>LTVNGDRLWDSLMDMAKIGPGIAGGNNRRTLTDEDAEGRRLFQRWCEAAGLTMGVDRMGTMFATRPGEDPEALPVYIGSHLDTQPTGGKFDGVLGVLAGLEVVRSLNDLNIKTKHPIVVTNWSNEEGARFAPAMLASGVFAGIHDLDYAYSRTDTDGKTYGEELKRIGWLGEEEVGARRMHAYFEYHIEQGPILEADGKQIGVVTHGQGLWWLEVTLTGKEAHTGSTPMAMRVNAGLAAARILEKVQEVAMAHQPGAVAGVGQMIFTPNSRNVLPGKVVFTIDLRTPSQAKLDSMRAIFEREVPAIAEELGVGCSIEAIGHFDPVTFDAVLVGRVRAAAERLGYSHMDIISGAGHDACWTARVAPSTMIFCPCVDGLSHNEAEEISPEWAAAGCDVLLHAVLETAEIVQ[2x]

N‐carbamoyl‐β‐alanine amidohydrolase (CβAA) constitutes one of the most important groups of industrially relevant enzymes used in the production of optically pure amino acids and derivatives. In this study, a CβAA‐encoding gene from Rhizobium radiobacter strain MDC 8606 was cloned and overexpressed in Escherichia coli. The purified recombinant enzyme (RrCβAA) showed a specific activity of 14 U·mg−1 using N‐carbamoyl‐β‐alanine as a substrate with an optimum activity at 55 °C and pH 8.0.

In this work, we report also the first prokaryotic CβAA structure at a resolution of 2.0 Å. A discontinuous catalytic domain and a dimerisation domain attached through a flexible hinge region at the domain interface have been revealed. We identify key ligand binding residues, including a conserved glutamic acid (Glu131), histidine (H385) and arginine (Arg291). Our results allowed us to explain the preference of the enzyme for linear carbamoyl substrates, as large and branched carbamoyl substrates cannot fit in the active site of the enzyme. The structural analysis provides new insights on enzyme–substrate interaction, which shed light on engineering of CβAAs for high catalytic activity and broad substrate specificity.> GPLGSSAPSVKGVSFDQANNLLIEPARIEEEELTLTILRQTGGLGISIAGGKGSTPYKGDDEGIFIS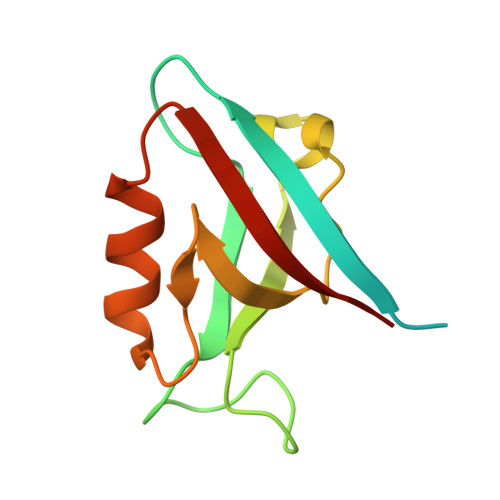RVSEEGPAARAGVRVGDKLLEVNGVALQGAEHHEAVEALRGAGTAVQMRVWRERM>[4x]MTMQGFGVHTSMWTMNWDRPGAERAVAAALKYEVDFIEIPMLNPPAV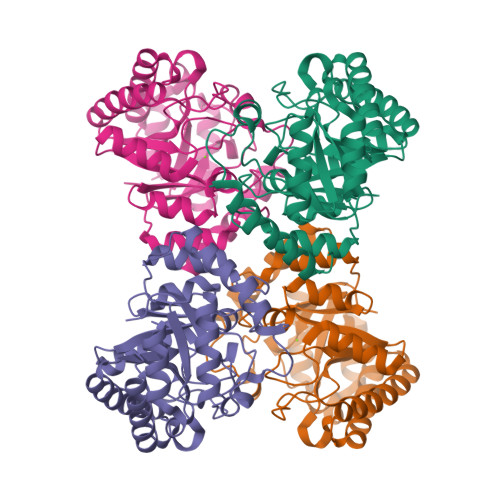DTEHTRALLEKNELRALCSLGLPERAWASVRPDAAIEHLKVAIDKTADLGGEALSGVIYGGIGERTGVPPTEAEYDNIARVLSAAAKHAKSRGIELGVEAVNRYENHLINTGWQAVQMIERVGADNIFVHLDTYHMNIEEKGVGNGILDAREHLKYIHLSESDRGTPGYGTCGWDEIFSTLAAIGFKGGLAMESFINMPPEVAYGLAVWRPVAKDEEEVMGNGLPFLRNKAKQYGLIGN> MSKKEININNYNDDAIQVLEGLDAVRKRPGMYIGSTDGAGLHHLVWEIVDNAVDEALSGFGDRIDVTINKDGSLTVQDHGRGMPTGMHAMGIPTVEVIFT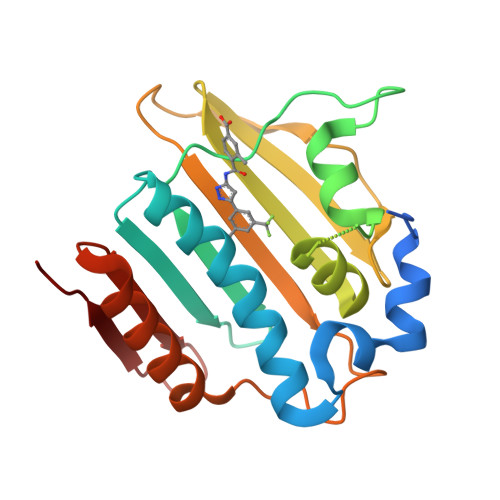ILHAGGKFGQGGYKTSGGLHGVGSSVVNALSSWLEVEITRDGAVYKQRFENGGKPVTTLKKIGTALKSKTGTKVTFMPDATIFSTTDFKYNTISERLNESAFLLKNVTLSLTDKRTDEAIEFHYEN We have identified a transporter from Syntrophobacter fumaroxidans (SfMCT) that shares 25 and 27% amino acid sequence identity, and 51 and 57% sequence similarity with the human SLC16 family L-lactate transporters MCT1 and MCT4. In summary, we reported two structures of the bacterial SLC16 homologue SfMCT in complex with the monocarboxylates TSA and L-lactate. We have presented the structures of an L-lactate transporter (SfMCT) with two different bound ligands. Both structures show SfMCT in the pharmacologically relevant outward-open conformation, which is an essential prerequisite for the design of L-lactate transport inhibitors using SfMCT structure-based homology models of human MCT1 and MCT4.

To understand the binding mechanism of L-lactate that bound to the purified, detergent-solubilized transporter with a Kd of 2.84 ± 0.15 mM, we co-crystallized SfMCT with its transported substrate. Two molecules of L-lactate (i.e., Lac1 and Lac2) were found in the binding pocket (see also Supplementary Fig. 5c,d for electron density and omit maps). The carboxylate group of Lac1 interacts with the Nη nitrogen atoms of the guanidinium group of R280 (TM8), while the hydroxyl group is hydrogen bonded to the hydroxyl group of Y119 (TM4). Furthermore, the carboxylate group of Lac1 is in hydrogen bonding distance to the hydroxyl group of Lac2. As observed for TSA, the Lac1 carboxylate group is sandwiched in the confinement formed by the side chains of L145 (TM5) and F335 (TM10). The phenyl-ring of F359 (TM11) points towards Lac1 with a distance of 3.4 Å between the C4 carbon atom of the benzene ring and the methyl-group of Lac1. Most residues involved in ligand binding adopt similar conformations in the SfMCT structures with bound TSA and L-lactate. The exception is L28 (TM1), which is rotated away from the central cavity in the presence of L-lactate. This removes the binding site obstruction observed in the presence of TSA and generates space to accommodate Lac2. Neither Y119A nor the conservative mutation Y119F showed any [14C]L-lactate transport, which is in line with our observation that the hydroxyl group of L-lactate interacts with the hydroxyl group of Y119 (TM4).

>[2x]MADQQTTMPRWVPLLLGLLGSTTCGMLLYAWSVFIKPLNAEFGWSRAEIAMAFAICCLIFGLMTFPAGRLSDKMGPRKVVMTGGVLLAIGFILSGFIQSKYQLYITYGVIAGFGGGMIYLPPIATAPKWWPDRRALATGFAVVGLGLGSFLMGPLATYIIEKPGMGWRYVFWYCGVAMGIMALIAGAFLEPPPAGWKPAGYTPPAPPAGAAAPKVTRDWTYEEAKGDTKFWLLYLAYFCGSFAGLMVIGHLAGFGRDAGLTAMAAAGAVSSLAFSNAATRILSGWFVDKIGIRVYFAALFALQTAAMIAIFQLGGSVVGLSIVAIVIGWNYGAMFTLFPATCLQFYGPTAQGSNYGLLFTACGLAGFAGPWVGGWLKDTTGTYYLPFLCAAALCALGTAIVFMTKPPEKKHALELEVLFQ> PQEEEMIHSILELEETPVREIMTPRVEMVAIEDEATLEDLLALYREHRYSRVPVYRESVDHIVGV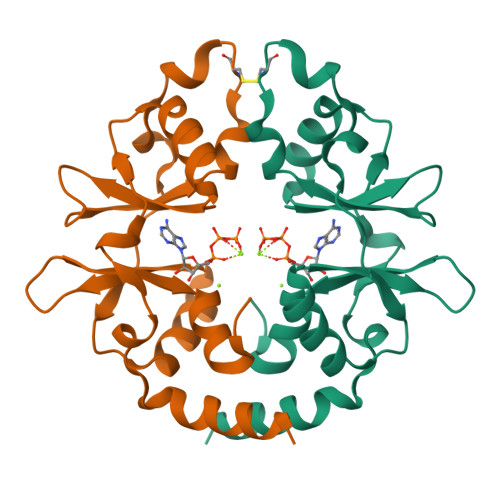AYAKDLLDYYCEEDLKGRTVASITHPPYFVPENMDAWSLLKELRRRKVHMAIVVDEFGGTAGLVTLEDVIEEIVGEI Flaviviruses use a ~70 nucleotide stem-loop structure called stem-loop A (SLA) at the 5′ end of the RNA genome as a promoter for RNA synthesis. Flaviviral polymerase NS5 specifically recognizes SLA to initiate RNA synthesis and methylate the 5′ guanosine cap. Here we report crystal structures of flavivirus SLA; DENV and ZIKV SLA were determined to 3.4 and 3.8 Å resolution, respectively. Both structures show similar structural elements, consisting of a top stem-loop, a side loop, and a bottom stem, but differ in size and the relative arrangements of the individual elements.

The DENV and ZIKV SLAs share ~58% sequence identity and are predicted to have similar ‘Y’-shaped structures, but ZIKV SLA shows different orientations of top stem-loop and side loop compared to DENV SLA. The ZIKV SLA is a 51 Å long by 65 Å wide, consisting of a top stem-loop (13 bp), a side loop (11 nt), and a bottom stem (11 bp). The top stem-loop helix is bent toward the bottom stem at a 46° angle, rendering ZIKV SLA a ‘V’-shaped molecule, rather than the ‘L’ shape observed for DENV SLA. The top stem-loop is extended by base pairs between 15GU16 and 46GC47, which were predicted to be in the bottom stem and the side stem-loop, respectively. The bulge (17GAA19), predicted to be between the top and bottom stem, does not exist, and is inserted in the extended top stem-loop. Because of base pairing between 15GU16 and 46GC47, the internal base pairs in the predicted side stem-loop (between 45AGC47 and 52GCU54) do not form, and the side loop of ZIKV SLA is single stranded. Surprisingly, the side loop also contains a previously unidentified, palindromic sequence (52GCUAGC57) that forms intermolecular Watson-Crick base pairs with equivalent region from the neighboring molecule. This side loop-side loop interaction in the ZIKV SLA dimer results in a dsRNA helix that is coaxially stacked, similar to the DENV SLA dimer. Hence, ZIKV SLA dimer also forms an unusual intermolecular 3-way junction structure where one helix is shared between two SLA molecules instead of the predicted intramolecular 3-way junction. When the DENV and ZIKV SLA structures are superposed by their conserved bottom stems, the top stem-loop helix and side loop of ZIKV SLA is related to the equivalent regions in DENV SLA by an approximately 180° rotation. This difference in orientation occurs because the bottom stem in ZIKV SLA is shorter than that in DENV SLA by 5 base pairs (16 bp vs. 11 bp), which corresponds to ~half-a-turn of a dsRNA helix, leading to an ~180° rotation of the top stem-loop.

> GCCCGGAUAGCUCAGUCGGUAGAGCAGCGGUAGCUGUUGAUCUGUGUGAAUCAGACUGCGACAGUUCGAGUUUGAAGCGAAAGCUAGCAACAGUAUCAACAGCUACCGCGGGUCCAGGGUUCAAGUCCCUGUUCGGGCGCCA>CGVGFIAAIDGKPRRSVVEKGIEALKAVWHRGAVDADGKTGDGAGIHVAVPQKFFKDHVKVIGHRAPDNKLAVGQVFLPRISLDAQEACRCIVETEILAFGYYIYGWRQVPINVDIIGEKANATRPEIEQIIVGNNKGVSDEQFELDLYIIRRRIEKAVKGEQINDFYICSLSARSIIYKGMFLAEQLTTFYPDLLDERFESDFAIYHQRYSTNTFPTWPLAQPFRMLAHNGEINTVKGNVNWMKAHETRMEHPAFGTHMQDLKPVIGVGLSDSGSLDTVFEVMVRAGRTAPMVKMMLVPQALTSSQTTPDNHKALIQYCNSVMEPWDGPAALAMTDGRWVVGGMDRNGLRPMRYTITTDGLIIGGSETGMVKIDETQVIEKGRLGPGEMIAVDLQSGKLYRDRELKDHLATLKPWDKWVQNTTHLDELVKTASLKGEPSDMDKAELRRRQQAFGLTMEDMELILHPMVEDGKEAIGSMGDDSPIAVLSDKYRGLHHFFRQNFSQVTNPPIDSLRERRVMSLKTRLGNLGNILDEDETQTRLLQLESPVLTTAEFRAMRDYMGDTAAEIDATFPVDGGPEALRDALRRIRQETEDAVRGGATHVILTDEAMGPARAAIPAILATGAVHTHLIRSNLRTFTSLNVRTAEGLDTHYFAVLIGVGATTVNAYLAQEAIAERHRRGLFGSMPLEKGMANYKKAIDDGLLKIMSKMGISVISSYRGGGNFEAIGLSRALVAEHFPAMVSRISGIGLNGIQKKVLEQHATAYNEEVVALPVGGFYRFRKSGDRHGWEGGVIHTLQQAVTNDSYTTFKKYSEQVNKRPPMQLRDLLELRSTKAPVPVDEVESITAIRKRFITPGMSMGALSPEAHGTLNVAMNRIGAKSDSGEGGEDPARFRPDKNGDNWNSAIKQVASGRFGVTAEYLNQCRELEIKVAQGAKPGEGGQLPGFKVTEMIARLRHSTPGVMLISPPPHHDIYSIEDLAQLIYDLKQINPDAKVTVKLVSRSGIGTIAAGVAKANADIILISGNSGGTGASPQTSIKFAGLPWEMGLSEVHQVLTLNRLRHRVRLRTDGGLKTGRDIVIAAMLGAEEFGIGTASLIAMGCIMVRQCHSNTCPVGVCVQDDKLRQKFVGTPEKVVNLFTFLAEEVREILAGLGFRSLNEVIGRTDLLHQVSRGAEHLDDLDLNPRLAQVDPGENARYCTLQGRNEVPDTLDARIVADARPLFEEGEKMQLAYNARNTQRAIGTRLSSMVTRKFGMFGLQPGHITIRLRGTAGQSLGAFAVQGIKLEVMGDANDYVGKGLSGGTIVVRPTTSSPLETNKNTIIGNTVLYGATAGKLFAAGQAGERFAVRNSGATVVVEGCGSNGCEYMTGGTAVILGRVGDNFAAGMTGGMAYVYDLDDSLPLYINDESVIFQRIEVGHYESQLKHLIEEHVTETQSRFAAEILNDWAREVTKFWQVVPKEMLNRLEVPVHL[6x];>QDFAEIYARFSDERANEQANRCSQCGVPFCQVHCPVSNNIPDWLKLTSEGRLEEAYEVSQATNNFPEICGRICPQDRLCEGNCVIEQSTHGAVTIGSVEKY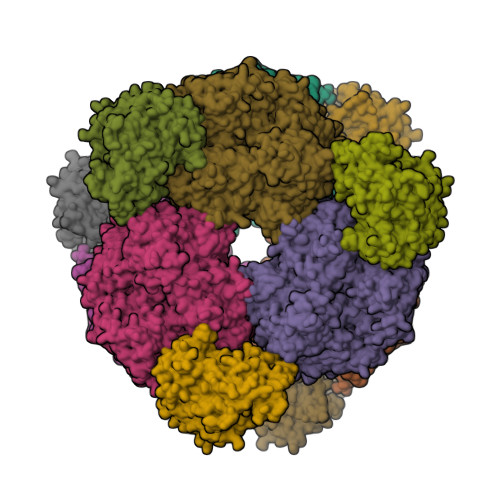INDTAWDQGWVKPRTPSRELGLSVGVIGAGPAGLAAAEELRAKGYEVHVYDRYDRMGGLLVYGIPGFKLEKSVVERRVKLLADAGVIYHPNFEVGRDASLPELRRKHVAVLVATGVYKARDIKAPGSGLGNIVAALDYLTTSNKVSLGDTVEAYENGSLNAAGKHVVVLGGGDTAMDCVRTAIRQGATSVKCLYRRDRKNMPGSQREVAHAEEEGVEFIWQAAPEGFTGDTVVTGVRAVRIHLGVADATGRQTPQVIEGSEFTVQADLVIKALGFEPEDLPNAFDEPELKVTRWGTLLVDHRTKMTNMDGVFAAGDIVRGASLVVWAIRDGRDAAEGIHAYAKAKAEAPVAVAAE[6x]> MAHHHHHHASPAPPPAAPSGQSGTYLFQDEFDGPAGSAPDASKWAVAKARETIKDPTYWERPENIGQYRDDRRNVFLDGKSNLVLRAAKNGPTYYSGKVQSLWRGGVGHTWEARIKLDCLTAGAWPAYWLGNDDQGEIDVMEWYGNGNWPSATTVHAKANGGEWKTHNIAVDSAWHTWRC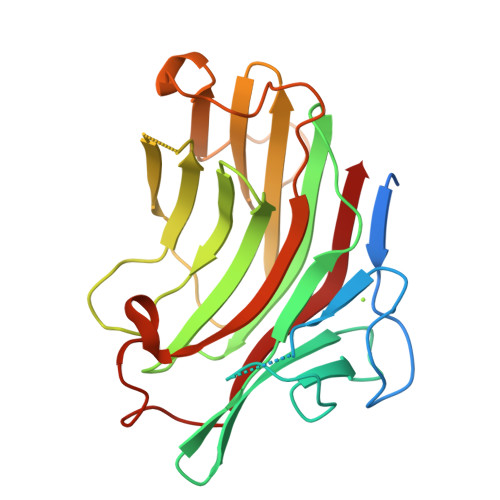QWDEAGIRFWKDYVDGAQPYFDVPASSLPDWPFNGPGYTVFPVFNLAVAGSGGGDPGPGSYPADMLIDWIRVW> GAMGTLTPKEAE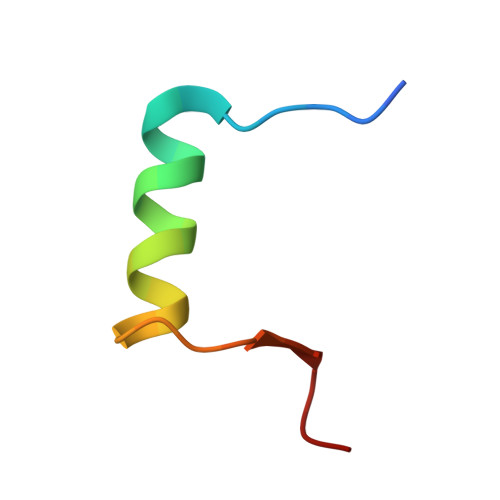LARRIRGAGGRTLNGFG>SMHLICQSGDVLSARYEIVDTLGEGAFGKVVECIDHKAGGRHVAVKIVKNVDRYCEAARSEIQVLEHLNTTDPNSTFRCVQMLEWFEHHGHICIVFELLGLSTYDFIKENGFLPFRLDHIRKMAYQICKSVNFLHSNKLTHTDLKPENILFVQSDYTEAYNPKIKRDERTLINPDIKVVDFGSATYDDEHHSTLVSTRHYRAPEVILALGWSQPCDVWSIGCILIEYYLGFTVFPTHDSKEHLAMMERILGPLPKHMIQKTRKRKYFHHDRLDWDEHSSAGRYVSRACKPLKEFMLSQDVEHERLFDLIQKMLEYDPAKRITL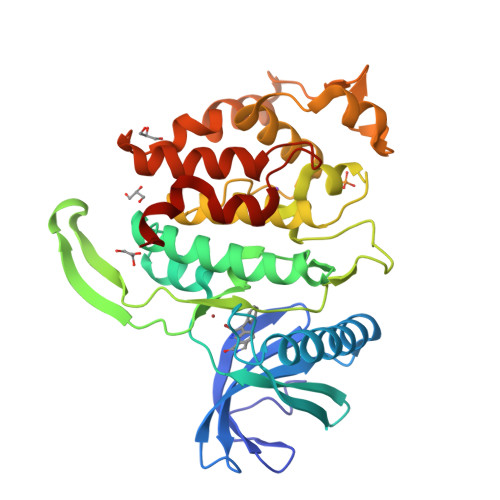REALKHPFFDLLKKSI[3x]> VHWTQEERDEIVKTFFSANSSA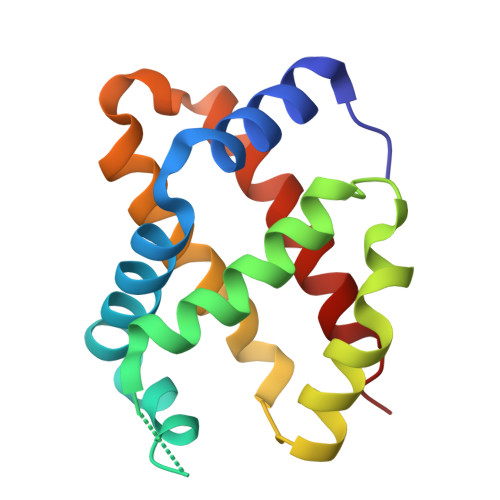IGTKALERMFVVFPWTNAYFAKXXXFSASIHAAIVVGALQDAVKHEDDVKAEFVNISKAHADKLHIDPGSFHLLTDSFIVELAHLKKVAFTPFVFAVWIKFFQVVIDAISSQYH> GHMNSFVGLRVVAKWSSNGYFYSGKITRDVGAGKYKLLFDDGYECDVLGKDILLCDPIPLDTEVTALSEDEYFSAGVVKGHRKES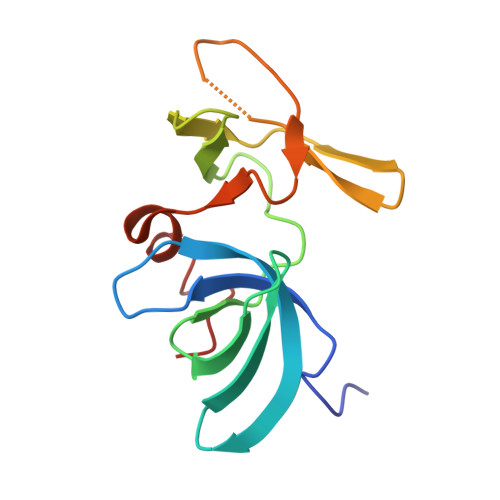GELYYSIEKEGQRKWYKRMAVILSLEQGNRLREQYGLG> MVSVIDKLVFDFGGKTLVSLAPDNNTLCVANKNGLTKILKTNNPEEEPETLDSSKLVSSIKCYSNSHFLMTTMQGDALRYNIDSSQEELLARFALPLRDCCVIHSGKMAVFGGDDLELILLELDDETHKKHAIKIDEQVSQISYNSQMNILAVSMINGKVQIFSLTSTIPNKVHELNDYIVANSYDDTHRDKILSNMMDDIDKDNDNDLSETADPDENNVADPEFCAANRICTRVAWHPKGLHFALPCADDTVKIFSIKGYSLQKTLSTNLSSTKAHFIDLQFDPLRGTYIAAVDLNNKLTVWNWETSEIHYTREFKRKITNIAWKIQADSKTLDLVLGTWSGSIAIVQNLAESVVSNIPDQSVAESSTKHGLFVDSESDLENLEGNDDINKSDKLFSDITQEANAEDVFTQTHDGPSGLSEKRKYNFEDEEDFIDDDDGAGYISGKKPHNEHSYSRVHKTHSFPISLANT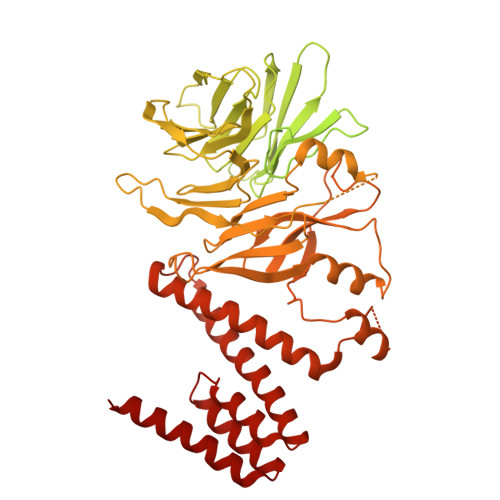GKFRYMPFSPAGTPFGFTDRRYLTMNEVGYVSTVKNSEQYSITVSFFDVGRFREYHFEDLFGYDLCFLNEKGTLFGQSKTGQIQYRPHDSIHSNWTKIIPLQAGERITSVAATPVRVIVGTSLGYFRSFNQFGVPFAVEKTSPIVALTAQNYRVFSVHYSQFHGLSYSLSELGTSSKRYYKRECPLPMSLPNINSDMKKDANLDYYNFNPMGIKSLFFSSYGDPCIFGSDNTLLLLSKWRSPEESKWLPILDSNMEIWKMSGGKETTDIHVWPLALAYDTLNCILVKGKHIWPEFPLPLPSEMEIRMPVFVKSKLLEENKAILNKKNEIGADTEAEEGEEDKEIQIPVSMAAEEEYLRSKVLSELLTDTLENDGEMYGNENEVLAALNGAYDKALLRLFASACSDQNVEKALSLAHELKQDRALTAAVKISERAELPSLVKKINNIREARYEQQLK> MFNRKRRGDFDEDENYRDFRPRMPKRQRIPPVVQLCKEMMPDIRTIGESVKAFEDDIKFLSEAIMNEYGHEDYFNNALLSTLNAVVVEQPQKQAAIALLTMVVNSKNNVAGKSIINYFFEELQKWCKQTYNDEFKSTSNETGPWNKIKLILRFLSILSPMFLVDELINIYKSLFELSIELNNLDPGNRVPLSEAIYTNTLLNIPYLFFFNRNNDGLRTKVEELLAYVEQNYLVKTTDINLLREYNGEPPYEMVELVRVVLPNVKKALINNLEQLNELFPDWNHLLTPQTGDEGFNDALTLPSVDDLKSFVRLNKNFGSVDSMWKTPRYAFHVYLPNSAGNFETVVPISTYAGQLFNDIIIDLVESLEFNRKEVARQVITLDLFFKAGIFTEPGESIAQLIATYEENPLAPTFKIEDLAIETILGLIFKLPSVSQPFAYFYTLLVDICQNSP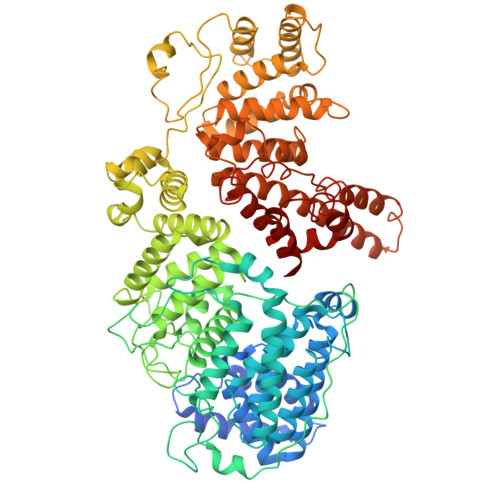KAIAPVFGRAFRFFYSHLDSLDFELKLRYLDWFSIQMSNFNFSWKWNEWEDDSIKFGKYFYNPKVNFAKNLIQKELRLTSNFSEVEDSLPQEFTKYLDTSYIPRDQLINYYQSLFTGYTVEEDSVRKNDLYFRQEGVPMENTVRKILDYTHKANNSREVTELESILGELKNEYGSIISDFNRFVIILLVQAVTDSGSRSLSHANKYINDLKEDLKTIFAKIELDIETKEYIIIEAVLTFWNANPQTGFLVADAFKYAGLLTSRTIFTFIFNETGLKNNGLIEATAIEAVFRNLSQQISEENESGNNFEFVFERLCTIANSTIDLLDVNADEDIEIPKVNGEMDIDDIEDDKLDLKWKYFTVIGFIKSILRRYSHEYRELADKFIANIDNAIPHESTRRTISNWIQETKEV CCs are quaternary structures comprising two or more α-helices supercoiled around each other with cyclic (Cn) or dihedral (Dn) symmetry. Here, we describe variants with all combinations of the aliphatic residues, Ile, Leu and Val, at a and d to give four classes of peptide: the ββ class, with a and d = Ile or Val; Lβ, a = Leu and d = Ile or Val; βL, a = Ile or Val and d = Leu; and LL, a = d = Leu. Peptides are named systematically appending the one-letter code for the amino acids at the a and d sites to “CC-Type2-“; e.g., CC-Hept becomes CC-Type2-LI. In summary, solution-phase data and X-ray crystal structures demonstrate conclusively that different classes of Type-2 coiled-coil (CC) peptides—i.e., based on abcdefg repeats with predominantly hydrophobic residues at a, d, e and g—adopt a range of distinct states.

As a = d = β-branched specify blunt-ended α-helical barrels, we explored all four combinations of Ile and Val at these sites. CC-Type2-VV, -IV, -VI and -II, were helical and bound DPH in solution consistent with α-helical barrels. Interestingly, X-ray crystallography revealed that oligomer state increased through this series: CC-Type2-VV was hexameric; CC-Type2-IV, heptameric; and CC-Type2-II, octameric. Concomitantly, the dimensions of the internal pore diameters increased: VV, 4.8–7.7 Å; IV, 6.2–9.2 Å; and II, 9.0–11.0 Å. Finally, the modelling offers a clear explanation for why the ββ and Lβ classes exclusively form non-collapsed Cn-symmetric α-helical barrels. Sequences from both classes scored worse when threaded onto most of the slipped and collapsed structures (upper-right-hand regions of Fig. 7e).

>XGEVAQAIKEVAKAIKEVAWAIKEVAQAIKGX[7x]> MSQDRKPIVGSFHFVCALALIVGSMTPFSNELESMVDYSNRNLTHVPKDLPPRTKALSLSQNSISELRMPDISFLSELRVLRLSHNRIRSLDFHVFLFNQDLEYLDVSHNRLQNISCCPMASLRHLDLSFNDFDVLPVCKEFG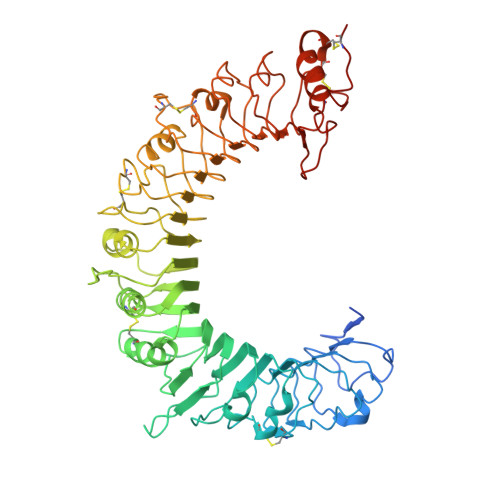NLTKLTFLGLSAAKFRQLDLLPVAHLHLSCILLDLVSYHIKGGETESLQIPNTTVLHLVFHPNSLFSVQVNMSVNALGHLQLSNIKLNDENCQRLMTFLSELTRGPTLLNVTLQHIETTWKCSVKLFQFFWPRPVEYLNIYNLTITERIDREEFTYSETALKSLMIEHVKNQVFLFSKEALYSVFAEMNIKMLSISDTPFIHMVCPPSPSSFTFLNFTQNVFTDSVFQGCSTLKRLQTLILQRNGLKNFFKVALMTKNMSSLETLDVSLNSLNSHAYDRTCAWAESILVLNLSSNMLTGSVFRCLPPKVKVLDLHNNRIMSIPKDVTHLQALQELNVASNQLKSVPDGVFDRLTSLQYIWLHDNPWDCTCPGIRYLSEWINKHSGVVRNSAGSVAPDSAKCSGSGKPVRSIICPTLVPR> M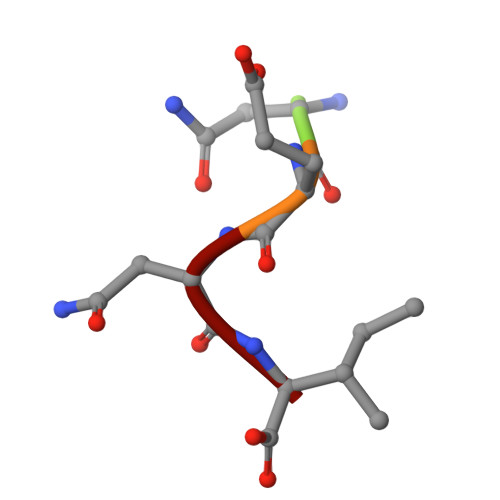NENI1-{2-fluoro-4-[(5-methyl-5H-pyrrolo[3,2-d]pyrimidin-4-yl)oxy]phenyl}-3-[3-(trifluoromethyl)phenyl]urea | C21 H15 F4 N5 O2 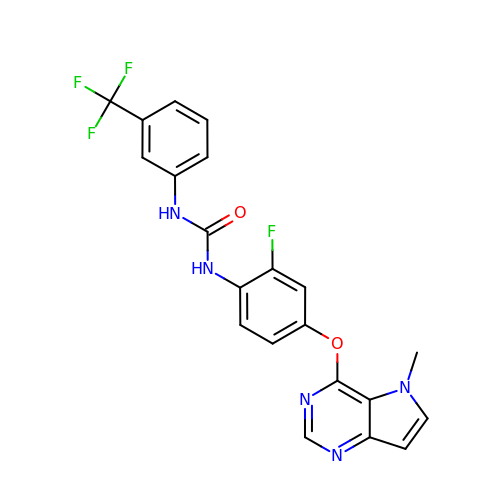| TWOLOZGQZKJZKJ-UHFFFAOYSA-N>[2x]MAAATGPSFWLGNETLKVPLALFALNRQRLCERLRKNPAVQAGSIVVLQGGEETQRYCTDTGVLFRQESFFHWAFGVTEPGCYGVIDVDTGKSTLFVPRLPASHATWMGKIHSKEHFKEKYAVDDVQYVDEIASVLTSQKPSVLLTLR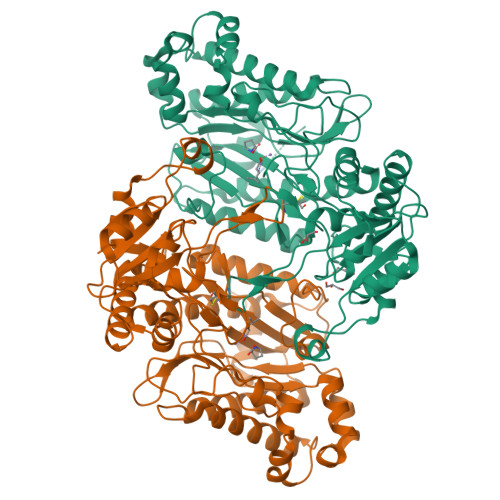GVNTDSGSVCREASFDGISKFEVNNTILHPEIVECQVFKTDMELEVLRYTNKISSEAHREVMKAVKVGMKEYELESLFEHYCYSRGGMRHSSYTCICGSGENSAVLHYGHAGAPNDRTIQNGDMCLFDMGGEYYCFASDITCSFPANGKFTADQKAVYEAVLRSSRAVMGAMKPGVWWPDMHRLADRIHLEELAHMGILSGSVDAMVQAHLGAVFMPHGLGHFLGIDVHDVGGYPEGVERIDEPGLRSLRTARHLQPGMVLTVEPGIYFIDHLLDEALADPARASFLNREVLQRFRGFGGVRIEEDVVVTDSGIELLTCVPRTVEEIEACMAGCDKAFTPFSGPK(1~{S},2~{S},3~{S},4~{S},5~{R},6~{S})-5-(hydroxymethyl)-7-azabicyclo[4.1.0]heptane-2,3,4-triol 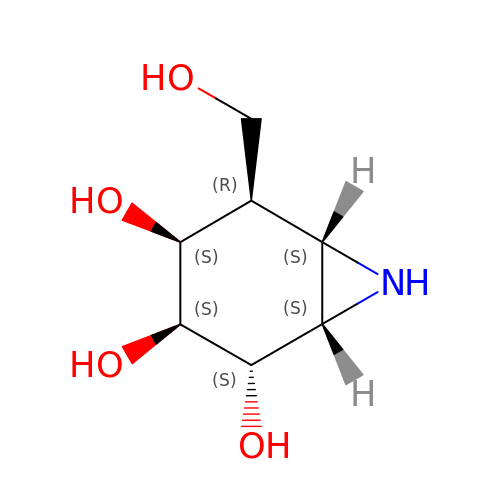| C7 H13 N O4 | GPIFFOGPRPKRHS-CLYCCYFHSA-N>[2x]LGTNYLLSGQTLDREGHLKNGDFDLVMQDDCNLVLYNGNWQSNTANKGRDCKLTLTDYGELVIKNGDGSTVWRSRAQSVKGNYAAVVHPD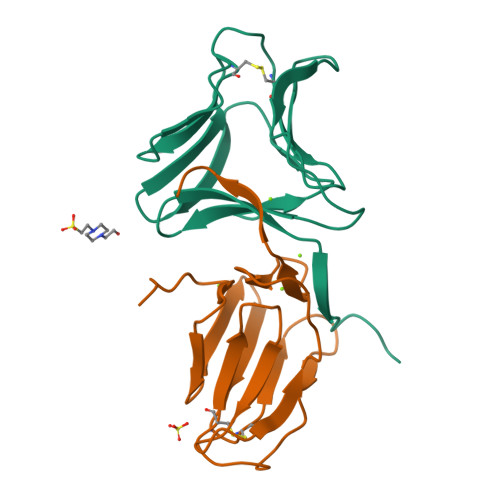GRLVVFGPSVFKIDPWVPG;>[2x]NIPFTNNLLFSGQVLYGDGRLTAKSHQLVMQGDCNLVLYGGKYGWQSNTHGNGEHCFLRLNHKGELIIKDDDFKTIWSSSSSSKHGDYVLILRDDGFAVIYGPAIWETSPQ> SDNIFVKPG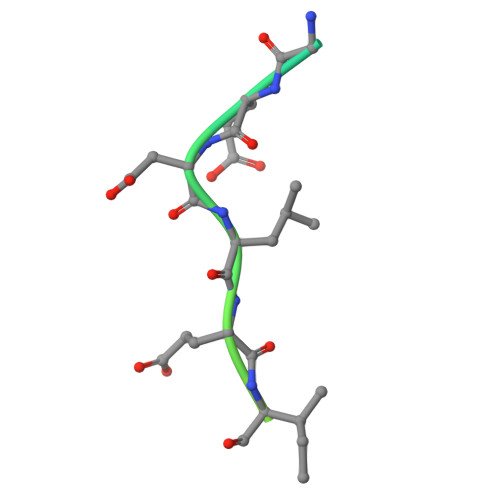EDLEIPLLSDYSDSENISEKS> SMTLTLNRQLLTSRQILVAFSGGLDSTVLLHQLVQWRTENPGVALRAIHVHHGLSANADAWVTHCENVCQQWQVPLVVERVQLAQEGLGIEAQARQARYQAFARTLLPGEVLVTAQHLDDQCETFLLALKRGSGPAGLSAMAEVSEFAGTRLIRPLLARTRGELVQWARQYDLRWIEDES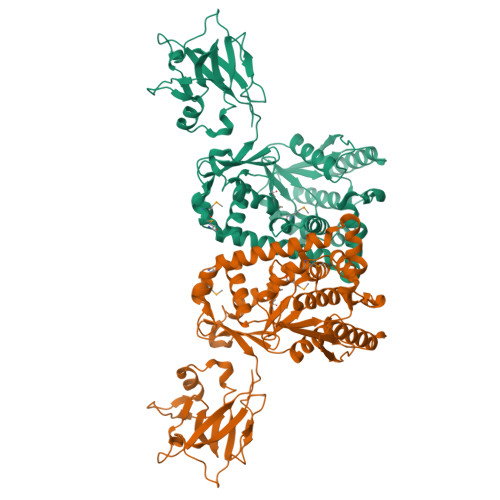NQDDSYDRNFLRLRVVPLLQQRWPHFAEATARSAALCAEQESLLDELLADDLAHCQSPQGTLQIVPMLAMSDARRAAIIRRWLAGQNAPMPSRDALVRIWQEVALAREDASPCLRLGAFEIRRYQSQLWWIKSVTGQSENIVPWQTWLQPLELPAGLGSVQLNAGGDIRPPRADEAVSVRFKAPGLLHIVGRNGGRKLKKIWQELGVPPWLRDTTPLLFYGETLIAAAGVFVTQEGVAEGENGVSFVWQKTLS> MIHCLRNIRTVSALQSKISYNLGGGNKRKKTSGDLDNYDVLFVGANLGGICSNHFDKDTHGKYKCFVSFDQPINQIYSVRIPYEQQRVRKSEYIHFSKKSINQFTPSEMLAVKEILPEQNAVVLSSGRRIGYNQLVLATGLKHDFSQIKGFYEALEHPEHPVYANRDPETWRSAQHKYSKYISNFKSGDGYFCIPEYPYAGEVECFNFFVSDEVWKWAQHHGALSPKHTFTIVNANEKFVHYCDSADAFIKERLEKRGIRVEYNTKLLEVHQDGQKATFINTKTGEKSVRDYNNLYSIVPS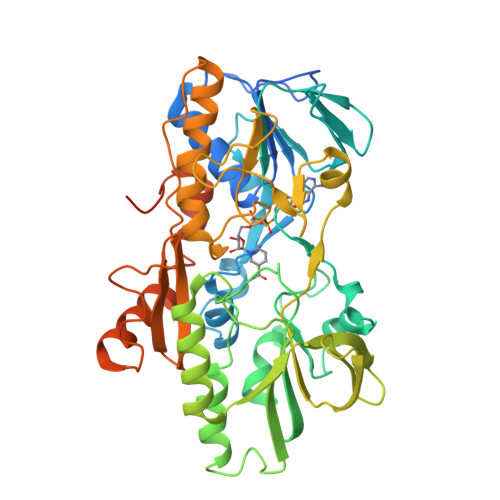KRQEFLDKAGLTNGNGLLNVDHQTLQHKKYKNIFGLGDAADLPTTKTFWAGWYQIAVVRNNVKRNLQGQTLNAHYDGFSKVPLFTGHQTLTYVAHSYGGVGNWQHLKHNNGGILAWMRYRSWAKGMAKKFQDFYNGARLGPPYHKVLKSFPELPGSPESQQSSGISKYFPTKTENKAAH> MMNDGKQQSTFLFHDYETFGTHPALDRPAQFAAIRTDSEFNVIGEPEVFYCKPADDYLPQPGAVLITGITPQEARAKGENEAAFAARIHSLFTVPKTCILGYNNVRFDDEVTRNIFYRNFYDPYAWSWQHDNSRWDLLDVMRACYALRPEGINWPENDDGLPSFRLEHLTKANGIEHSNAHDAMADVYATIAMAKLVKTRQPRLFDYLFTHRNKHKLMALIDVPQMKPLVHVSGMFGAWRGNTSWVAPLAWHPENRNAVIMVDLAGDISPLLELDSDTLRERLYTAKTDLGDNAAVPVKLVHINKCPVLAQANTLRPEDADRLGINRQHCLDNLKILRENPQVREKVVAIFAEAEPFTPSDNVDAQLYNGFFSDADRAAMKIVLETEPRNLPALDITFVDKRIEKLLFNYRARNFPGTLDYAEQQRWLEHRRQVFTP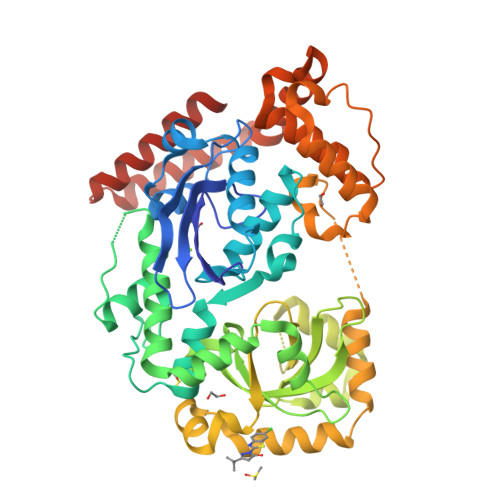EFLQGYADELQMLVQQYADDKEKVALLKALWQYADEIVEHHHHHH> HHHHHHGSAQLPSPTNGKKWEKVEQLSDEFDGNSIDTNKWYDYHPFWEGRAPSNFKKGDAFVSD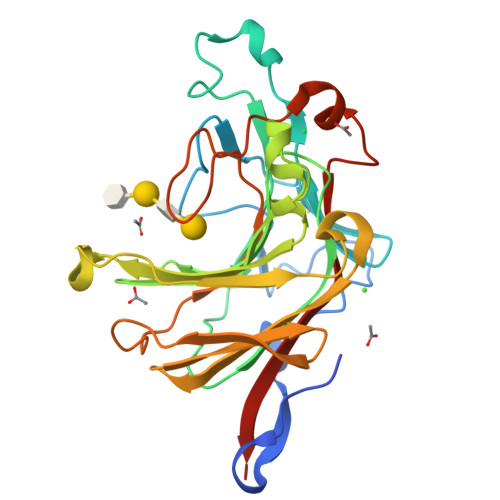GFLNLRSTLRKEPSSVQDPFKDIWVDAAAAVSKTKAQPGYYYEARFMASSLSMTSSFWFRVGQFSSIDVIEHIGDPSKENRQDDLPYQYHVNTHYYGKHAGLQPLGTEYKMPGRGRDNFYTYGFWWKSPNELLFYFNGKQVMRIVPRVPLDEELRMIFDTEVFPFATAGVANIGLPKPENLRDNSKNTMKVDWVRVYKLVDGTA> MRGSHHHHHHGSHQLTIVHLEARDIDRPNPQLEIAPKEGTPIEGVLYQLYQLKSTEDGDLLAHWNSLTITELKKQAQQVFEATTNQQGKATFNQLPD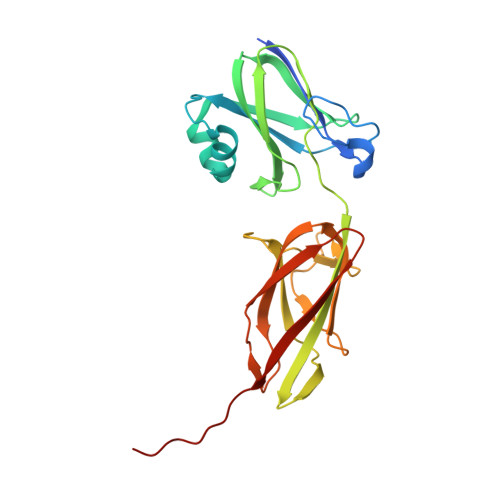GIYYGLAVKAGEKNRNVSAFLVDLSEDKVIYPKIIWSTGELDLLKVGVDGDTKKPLAGVVFELYEKNGRTPIRVKNGVHSQDIDAAKHLETDSSGHIRISGLIHGDYVLKEIETQSGYQIGQAETAVTIEKSKTVTVTIENKKVPTPKVPSR> MSDEKKILGEERRSLLIKWLKASDTPLTGAELAKRTNVSRQVIVQDVSLLKAKNHPILATAQGYIYMKEANTVQAQRVVAC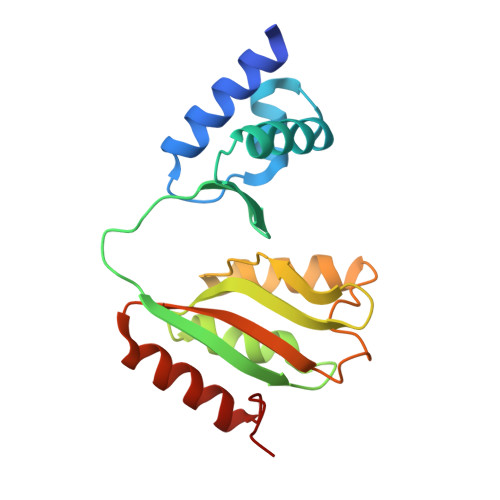QHGPADMKDELLTLVDHGVLIKDVTVDHPVYGDITASLHLKSRKDVALFCKRMEESNGTLLSTLTKGVHMHTLEAESEAILDEAIRALEEKGYLLNSF>SNAMKNEHTTLLVIGGGPGGYVAAIRAGQLGIPTVLVERDRLGGTCLNIGCIPSKALIHVADAFEQACGHAGEGALGIRVRAPEIDIAKSVAWKDGIVDRLTRGVGALLKKSGVRVLHGEARVIDGKTVEVVSAGHAVRIGCEHLLLATGSEPVELPSMPFGGHVVSSTDALSPATLPKRLVVVGAGYIGLELGIVYRKLGVDVSVVEAAERVLPAYDAELVRPVADSLARLGVRLWLGHKVLGLDKHGAVRVQAADGAEQTLPADRVLVAVGRRPRVDGFGLETLMLDRNGRALRIDDTCRTSMRNVWAIGDVAGEPMLAHRAMAQGEMVAELIAGRRRQFMPAAIPAVCFTDPEIVTAGWSPDDAHAAGVDCLSASFPFAANGRAMTLQATDGFVRVVARRDNHLIVGWQAVGRGVSELAAAFSQSLEMGARLEDIGGTIHAHPTLGEALQEAALRALGHALHV[4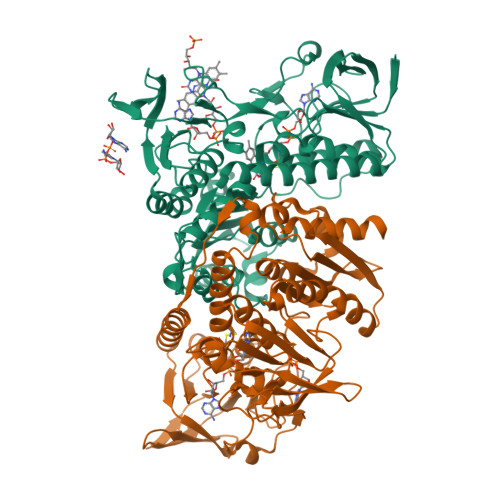x]> SGRPMPVFEDVTRALVRELNPRG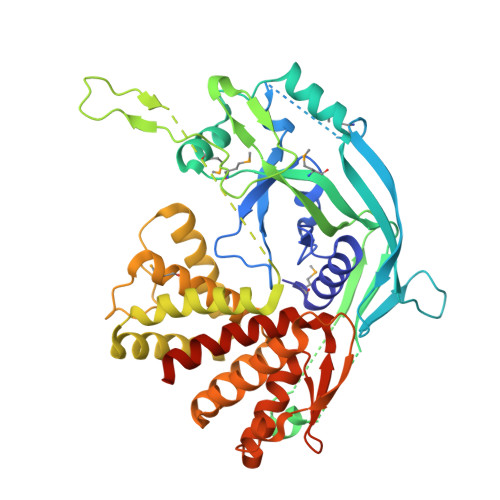DLTPLDSLIDFKHFRPFCLVLRKRKSTLFWGARYVRTDYTLLDLLEPGSSPSDLTDSGNFSFKNMLDVQVQGLVEVPKTVKVKGTAGLSQSSTLEVQTLSVAPSALENLKKERKLSADHSFLNEMRYHEKNLYVVMEAVEAKQEVTVEQTGNANAIFSLPSLALLGLQGSLNNNKAVTIPKGCVLAYRVRLLRVFLFNLWDIPYICNDSMQTFPKIRRVPCSAFISPTQMISEEPEEEKLIGEMHEDFKTLKEEVQRETQEVEKLSPVGRSSLLTSLSHLLGKKKELQDLEQKLEGALDKGQKVTLEALPKDVLLSKDAMDAILYFLGALTELTEEQLKILVKSLEKKILPVQLKLVESTLEQNFLQDKEGVFPLQPDLLSSLGEEELTLTEALVGLSGLEVQRSGPQYAWDPDTRHNLCALYAGLSLLHLLSRKSNALTYCALS> VIG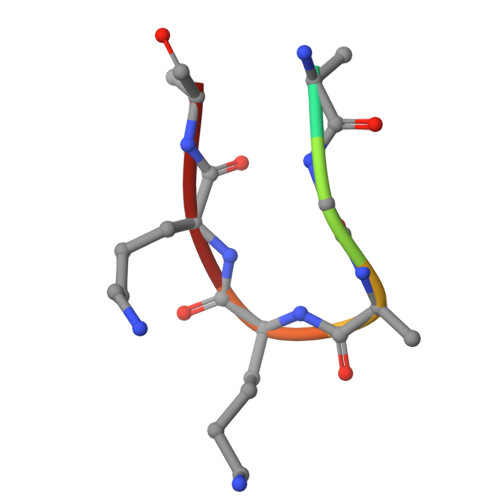AKKA> MKTEWPELVGKSVEEAKKVILQDKPAAQIIVLPVGTIVTMEYRIDRVRLFVDKLDNIAQVP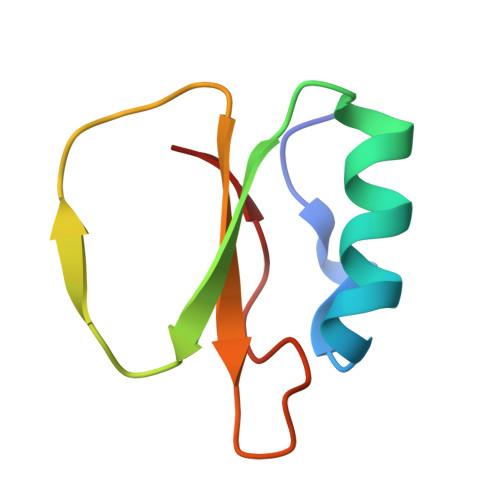RVG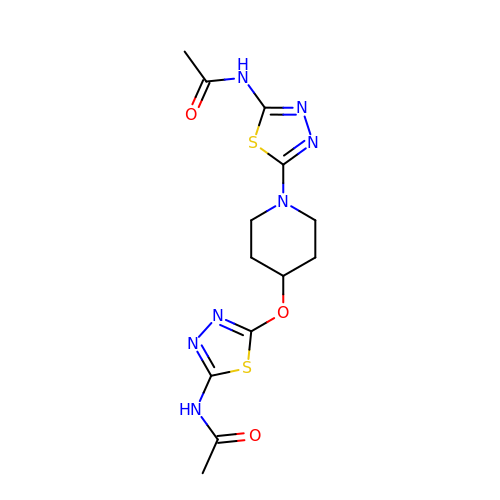N-[5-(4-{[5-(acetylamino)-1,3,4-thiadiazol-2-yl]oxy}piperidin-1-yl)-1,3,4-thiadiazol-2-yl]acetamide | C13 H17 N7 O3 S2 | UTGXSPFIBVKMDL-UHFFFAOYSA-N>[4x]SNAMNSTIQTILGHRSIRKFTSQPIDKEQLETILQAGLAASSSSMLQVVSI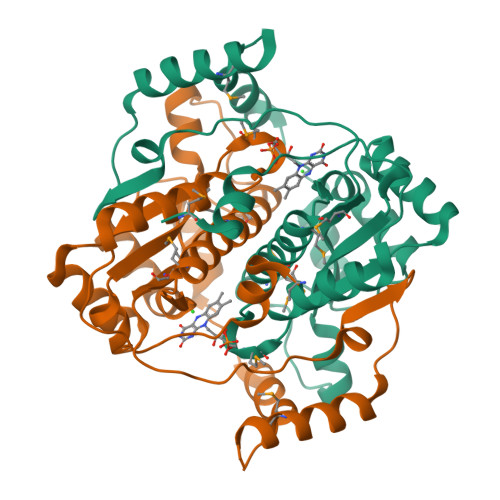VRVTDIEKRSQLAKFAGNQAYVESAAEFLVFCIDYQRHASINPDVQADFTELMLIGAVDSGIMAQNCLLAAESMGLGGVYIGGLRNNAQQVDELLGLPQNTAILFGMCLGHPDQNPEVKPRLPAHVVVHENQYQDLNLDDIQAYDQTMQNYYANRSSNQKQSTWSQEVTSKLAGESRPHILPYLNGKGLAKK> MHHHHHH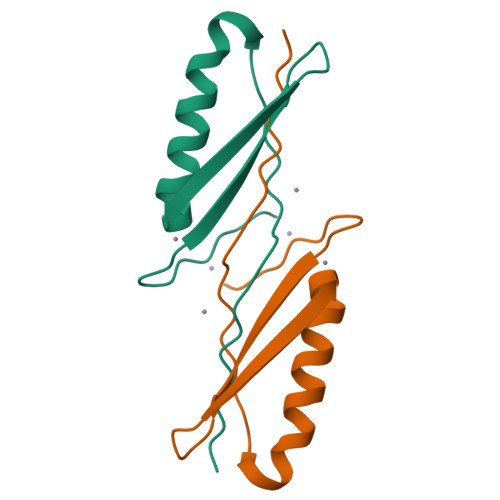AMEEVTIKANLIFANGSTQTAEFKGTFEKATSEAYAYADTLKKDNGEWTVDVADKAYTLNIKFAG> M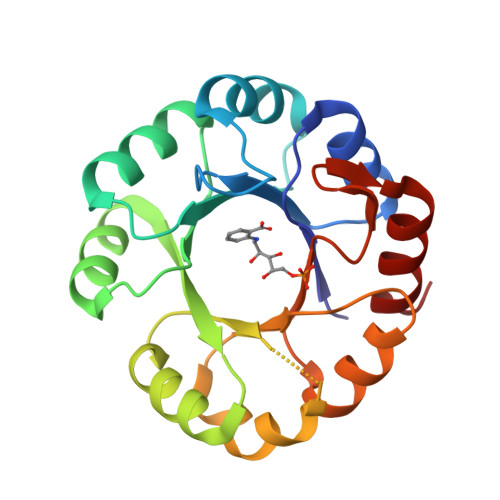VRVKICGITNLEDALFSVESGADAVGFVFYPKSKRYISPEDARRISVELPPFVFRVGVFVNEEPEKILDVASYVQLNAVQLHGEEPIELCRKIAERILVIKAVGVSNERDMERALNYREFPILLDTKTPEYGGSGKTFDWSLILPYRDRFRYLVLSGGLNPENVRSAIDVVRPFAVDVSSGVEAFPGKKDHDSIKMFIKNAKGL>[4x]ETGQVAASPSINVALKAAFPSPPYLVELLETAASDNTTIYYSLLDRIAKGHFAEATTDKALYEKFLEVLRDDGHMDPEALSAFKLALSLRTATPRVEAHYQYYTATVEPSLSGTQEGCDQWFLIDGEQYCSPTLDTSHGKVKGEDQLRTLPFDRKFGVGSRDVILYADITSKSFAPFHEVAMDLAKKGKASYRVRYRRSPSHSRESLSVNGYGVELVLKRTDYIVIDDRDTGAAAKPAEENDQKPLVGHETVLDDGEEIADIKPLEKSELAALGMKAASFVMQSEKPFEALLKLTQDFPKYSNSLGSQNVSAEFEAEHRGNREVFLPEGSNVLWLNGLHLIDRQIQPFGLVDLLTRERKLIKSVLDLGLTGQQAVDLLGHAEVAHAKSGDDEPRRFALSRRNTLIFPEDKNELTVLNVNKIYIENHDLMSKVPVIEASKESTRDDWAALTVVADLDDIEGQELVYYALRFRKSNDGVRLDI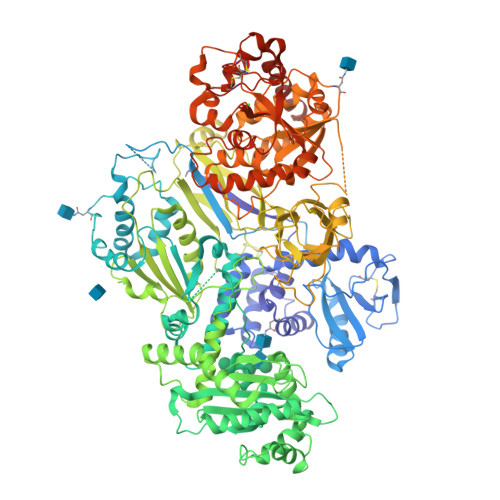VHNPKDTSRSPSVLAQRLKSREDKLLDFTRFLDLETALETGEFEPDVAYDASLANFLASSNMKAGDNFVILNGRVLGPITSADDFKKEDFEVFLQAERRTRILPVYKALEDLGLDDKVSGPLSAAKLTSVTALSTISDLPQGIFDNAPTVRTTLFKQWNSTYTSFEVGDASTATIFFVAVINPASEIGQRWVAVLKVLSELEGVHLRVFLNPTVMIEELPVKRFYRYVLSSSPSFDESGKVKALSARFTGVPRETLLVVGMDVPPAWLVTSKVAVDDLDNLRIKDIKAKRGTEHVEAIYELEHILIEGHSREIPGAHAPRGVQLVLETENNPHFADTIIMANLGYFQFKANPGVYNIRLKEGRSSEIFTLESVGAKGWGPIPGDDNTEVVLMDFQGTTLYPRLRRKPGMEEEDVLEPSTKSGEESGSGARNLVSRGIKFAEGLLGRGNKAAEATKSVSKTEHAEINIFSVASGHLYERMLNIMMASVMHHTNHTVKFWFIEQFLSPSFKDFIPHMAAEYGFKYEMVTYKWPHWLRQQKEKQREIWGYKILFLDVLFPLSLDKVIFVDADQIVRTDMYDLVEHPLDGAPYGFAPMCDSRVEMEGYRFWKTGYWANYLKGKPYHISALYVVDLQRFRELAAGDRLRQQYHALSADPNSLANLDQDLPNHMQFTIPIATLPQEWLWCETWCSDETLKDARTIDLCNNPMTKEPKLDRARRQVPEWTKYDEEIAELARRVREEKPKKKEEEKVQKNPKSRRLDGDEEEVKTVREGTKHHHHHH Like MhFbpA and Thermus thermophilus FbpA (TtFbpA), McFbpA adopts a typical fold of class III periplasmic iron binding protein with the two globular lobes. Similar to other FbpA structures, McFbpA has two globular α/β domains named the N terminal lobe (Asn1-Trp95 and Val235-Val273) and the C terminal lobe (Tyr107-Ala221 and Thr274-Lys312). Each of the lobes consists of α helices surrounding a twisted mixed β sheet in the center. These two lobes are connected by a pair of antiparallel β strands (Phe96-Phe106 and Gly222-Val234), which acts as a hinge allowing for the adoption of either the open or closed conformation. Isogenic mutants of FbpA and AfeA were constructed, demonstrating that FbpA is essential for the utilization of human Tf and Lf as iron sources and that AfeA does not take up iron from these iron sources.

Two crystallization conditions were identified within 1 week after setup, producing the apo (colourless) and the holo (red–orange) crystal forms. Our structural studies yielded the structure of M. catarrhalis FbpA in two different forms: an apo open form and an iron-holo open form. Comparisons with other FbpAs indicate that both iron-holo and apo McFbpA in this study are in the open conformation. Two high resolution crystal structures of the M. catarrhalis FbpA were solved in the iron-holo open and apo open conformations, revealing more details about the mechanism behind FbpA-mediated iron transport. The process of how iron is bound in a class III FbpA has been proposed in studies with T. thermophilus FbpA (TtFbpA). The proposed mechanism of iron binding with insights from both the previous study and the current study is illustrated in Fig. 7. The synergistic anion (e.g., carbonate) binds to the open FbpA through the arginine residues in N terminal lobe (Step 1). The ferric ion then binds to the three tyrosines in the C terminal lobe (Step 2) which results in the FbpA adopting a closed conformation through bidentate binding of iron by the carbonate anion (Step 3).

>NEIVVYSARADELLKPIAEAYQQKTGTKVTVVSDKAGPLMERLKAEGKNTQADVLITVDGGNLWQATQAGVLRPINSSVLKSNIPSHLRDPKNHWFGLSVRARTIFYNPNKVNPSELSTYADLADPKWKGRLCLRTSNNVYNQSLVATMIANHGQATTDRVVKGWVANLAAAPFANDTALLEAIDAGRCDVGIANTYYYGRLLNSKPQVANNVKVFFANQAGKGTHVNVSGAGVVKHSDNPAEAQKFIEWLSSNEAQRLYADRNFEYPANIQVTPTPAVARWGRFKQDFINVSVAGQNQQKAIMTMKRAGYK[4x]>SVKTGIYQVLNGSRLCIKAEMGIQLIVQDKESVFSPRRYFNIDPNATQASGNCGTRKSNLLLNFQGGFVNLTFTKDEESYYISEVGAYLTVSDPETVYQGIKHAVVMFQTAVGHSFKCVSE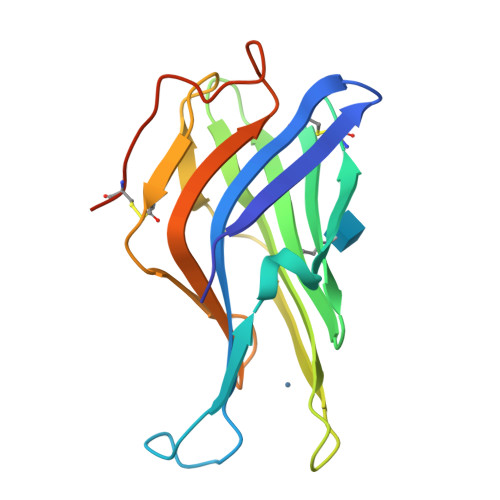QSLQLSAHLQVKTTDVQLQAFDFEDDHFGNVDECSSDYTHHHHHH[2x]> MASDMEEKFREAFILF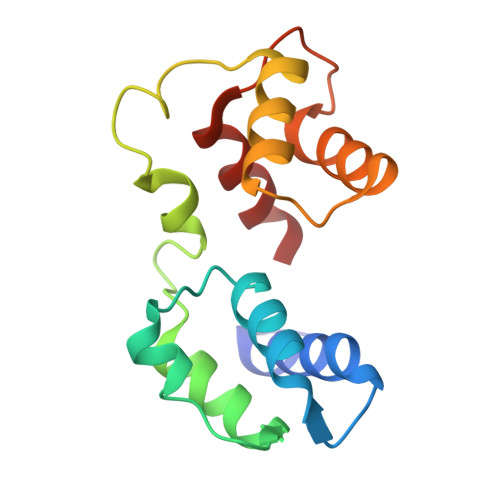SSCSDHIEMYKFFELMNSFGIILTNDEKAALPNDINMDYWLNFAKKHYNYEQPFKHINNVNEQNTNVQIKIDNFLGIMKALDTRLTESDLNILLQITNPENKTTLNLKTVSQKLTESI2-[[4,6-bis(azanyl)-2,2-dimethyl-1,3,5-triazin-1-yl]oxy]-N-(4-chlorophenyl)ethanamide 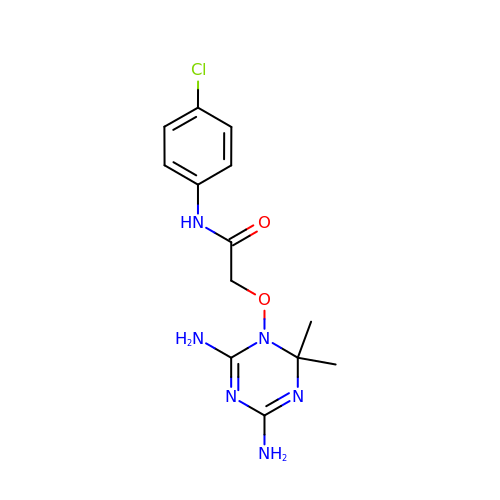| C13 H17 Cl N6 O2 | NFSDKWLTDMRPDV-UHFFFAOYSA-N> GSHMEKLAKNKVISIDAGRKY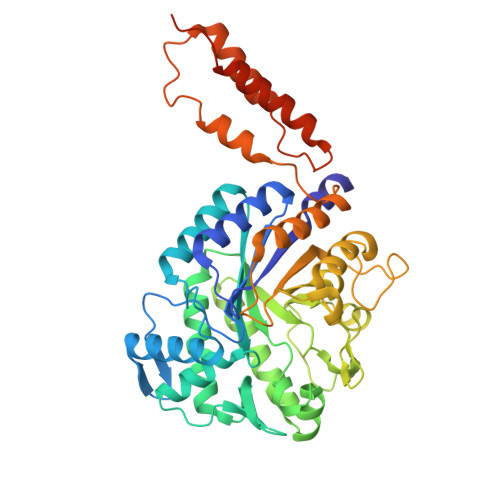FTLNQLKRIVDKASELGYSDVHLLLGNDGLRFLLDDMTITANGKTYASDDVKKAIIEGTKAYYDDPNGTALTQAEVTELIEYAKSKDIGLIPAINSPGHMDAMLVAMEKLGIKNPQAHFDKVSKTTMDLKNEEAMNFVKALIGKYMDFFAGKTKIFNFGTDEYANDATSAQGWYYLKWYQLYGKFAEYANTLAAMAKERGLQPMAFNDGFYYEDKDDVQFDKDVLISYWSKGWWGYNLASPQYLASKGYKFLNTNGDWYYILGQKPEDGGGFLKKAIENTGKTPFNQLASTKYPEVDLPTVGSMLSIWADRPSAEYKEEEIFELMTAFADHNKDYFRANYNALREELAKIPTNLEGYSKESLEALDAAKTALNYNLNRNKQAELDTLVANLKAALQGLKPAVTHSGSLDENEVAANVETRP>[3x]MSFVEDYLTKLQERPTIIENPNILKGSKIFNAIYRVDDFVYIHIQSIKSEDGYNQYNVIEPPRPTHDE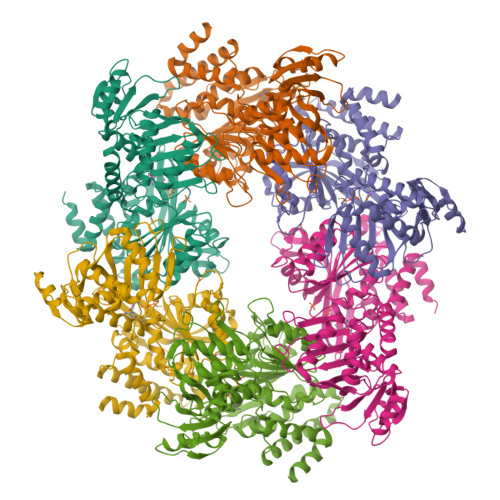MEEIEEKFALSIGDKEPPEDTKEKEKLIRSILDKILLRMRLSVPKEYVIYHFIRDKLYTGSLEPLIRDPYIEDISIPGLGHVYIVHKVFGPMRTSIKFENYEELDNLIVSLSEKSYRPVSHNRPVVDASLPDGSRVNFVYGVDISRRGSNLTVRKFSRVPTSITQLIMFGTLSSMMAAYIWTMLDEGMNLFVCGETASGKTTTLNAITAFIPPNLKIVTIEDTPELTVPHSNWVAEVTRETGGEGTIKLFDLLKAALRQRPNYILVGAIRDKEGNVAFQAMQTGHSVMATFHAANITTLIQRLTGYPIEVPKSYINNLNIALFQTALYDKKGNLIRRVVEVDEIIDIDPVTNDVVYIPAFTYDSVQDKMLFAGKGSSYLIENKIAVKRGIDRRNIGLLYDELQMRSRFLNLLVEKKIFNYYDVWDYILRARQMGLEEAIKYVSNI Through a systems-based approach, here we show that the symbiont Bacteroides uniformis deploys a single, exemplar polysaccharide utilization locus (PUL) to access yeast β(1,3)-glucan, brown seaweed β(1,3)-glucan (laminarin), and cereal mixed-linkage β(1,3)/β(1,4)-glucan. As exemplified by the β(1,3)-glucan utilization loci (1,3GULs) elucidated here, PULs encode concerted molecular systems of surface glycan binding proteins (SGBPs), carbohydrate-active enzymes (CAZymes), TonB-dependent transporters (TBDTs), and sensor/regulators to recognize, capture, import, and saccharify individual substrates. (ii) BuGH158 is a strictly specific, retaining endo-β(1,3)glucanase with a triose phosphate isomerase (TIM) barrel fold. Whereas BuGH158 is a highly specific laminarinase, BuGH16 is a generalist endo-β(1,3)-glucanase that can accommodate backbone β(1,4)-glucosyl linkages (as in MLG) and long/frequent β(1,6)-glucosyl branches (as in EbLam and yBG).

BuGH158 consists of an N-terminal (α/β)8 TIM barrel domain and a C-terminal, eight-stranded immunoglobulin (Ig)-like domain in contact with helices α7 and α8 of the TIM barrel. Additional loops contribute to the extensive contact between domains, with one from the Ig-like domain extending above the TIM barrel to shape the active-site cleft. A Dali structure similarity search returned members of clan GH-A as the top 20 structural homologs (Table S4 at the URL mentioned above), confirming the bioinformatics prediction that GH158 constitutes an evolutionarily distinct family within this clan. Clan GH-A members present the conserved catalytic acid/base and nucleophile residues on loops immediately following strands β4 and β7, corresponding to E137 and E220, respectively, in BuGH158. Additionally, a conserved asparagine (N136) precedes the general acid/base (E137) and is anticipated to engage in hydrogen-bonding interactions with the substrate. Indeed, site-directed mutation of N136, E137, or E220 to alanine completely abolished catalytic activity (data not shown). The active-site cleft surrounding the catalytic sidechains is rich in surface-exposed aromatic residues oriented to engage in stacking interactions with the substrate. Crucially, this superposition also reveals that 6-OH of the glucosyl residue in the −1 subsite is oriented toward a pocket lined with aromatic residues that may accommodate a single β(1,6)-linked glucose branch in BuGH158. Indeed, a glucosyl residue could easily be manually docked into this position without clashes. This structural feature provides a plausible explanation for the strict LdLam specificity and poor activity on yBG, the latter of which contains longer β(1,6)-linked glucose branches.

>[2x]AMGIVIEKAADGYKLSIDGRETYIKGVGGTYRLDIAAQSGANAFRTWGGNVEEIKKNLALASEHNMYVMQGIGMTKDSIRYYDDEYKNKMREEVRLLAETFKNDTSLLAWGIGNEIELGNANIAAAWNFVEELAQLIKSIDKRHLVSTVISYNPSALDSVAKYAPSLDYVGINVYGPMGEVQAVVDRSDYKGAFMITEWGPTGWWETASTEWKAPIEQTSEEKRQVYEERYTQYISANTRCLGSFVFLWGQKEERTPTWFSMFVEDKVDSLPLKGEKTPMVEAMQRVWTGKELDETAPIVRGMTIDGKSAIDNVRIKAGTLFKAEVSVTDKENDSLAYVWEVLKEATVLGFGGSYEPRPERMGDVAVSDKNVYETMIKVPGEYRLYVYVLDNTGFVSTANIPFQVID>[2x]MQNPKLGVSPIQDVINAMTLDEKIQLVVGSSGKYESQMEATIGNQGQLVQGAAGQVNGIERLGIPATVVADGPAGLRIDPKRKNTDKTFYCTHFPVATVMSSTWNKDLVYSVGTSMGDEVKHYGVDVLLAPATNIMRNPLCGRNFE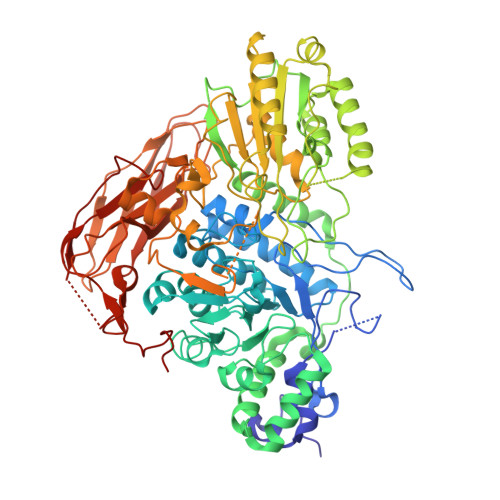YYSEDPLLAGTICAAMVNGIESNDVGTSLKHFALNNQETNRTRNNVIGNPRTFREIYLKPFEIVIKEAQPWTVMTSYNLINGTMSSERCDLITEILRHEWGFKGMVMTDWFGGISAAAQMEAGNDLLMPGKADQVKEIRKAVLNGRLSMEILDRNVRHILEYIMQTPRFKQYVADNNPDLKGHALVARNAATEGMVLLKNNKNVLPLVQKIKNIALFGNTSYDFIAGGTGSGNVNHAYVVSLLDGLKNAGYQVDGDIQKSYIEYAPKAKANLPKPKNPLEAFLPGHFIPEMSLAELNMSAAVKNNDLAIITIGKSSGEFLDRKISDSFNLTKEEKDMISGVCNAFHKAGKKVVVILNVCGVIETKSWIGGPDAVLLSWLPGQEGGNCVADILTGKENPSGRLPMTWPVSYNDVPSKADFPNPETVKVDDVLGMFMGKGIGSKGDVKNVDYTEYNDGVYVGYRYYQTKNVPVSFPFGYGMSYTTFKYGKPVVTKDAQGNIKVLVTVKNAGKVAGKEVVQVYVAAPGKDMDKPAKELRGFAKTKKLQPGESETVTIDIPYKNLASFNEVDSQWQVEAGNYKVMVAKNAADLKPLTTVITEEAGVTEKVRPCLLKEVK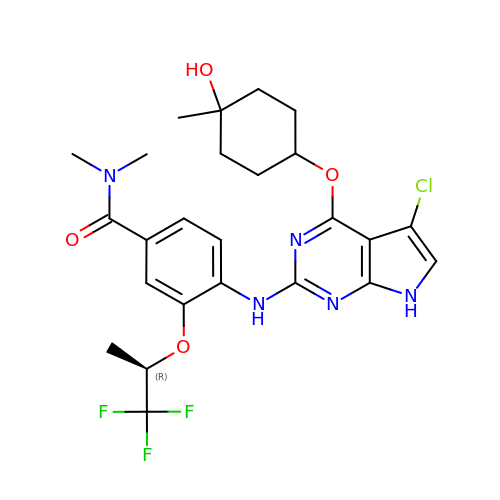4-({5-chloro-4-[(cis-4-hydroxy-4-methylcyclohexyl)oxy]-7H-pyrrolo[2,3-d]pyrimidin-2-yl}amino)-N,N-dimethyl-3-{[(2R)-1,1,1-trifluoropropan-2-yl]oxy}benzamide | C25 H29 Cl F3 N5 O4 | IUWWRSQCDUQDEZ-CAQPCFEESA-N> GLYLQVGAFANPD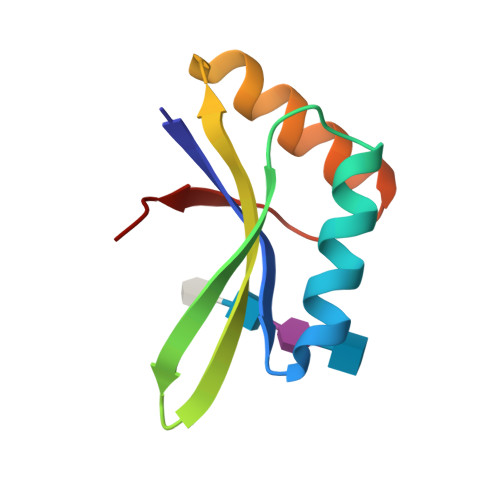AAELLKAKLSGVTAAPVFISSVVRNQQILHRVRLGPIGSADEVSRTQDSIRVANLGQPTLVRPD>[4x]HYTWPRVNDGADWQQVRKADNWQDNGYVGDVTSPQIRCFQATPSPAPSVLNTTAGSTVTYWANPDVYHPGPVQFYMARVPDGEDINSWNGDGAVWFKVYEDHPT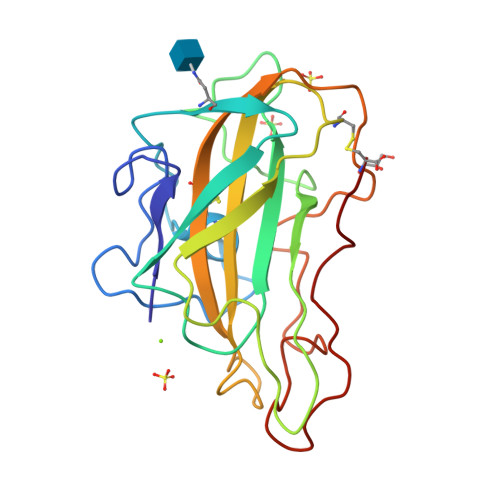FGAQLTWPSTGKSSFAVPIPPCIKSGYYLLRAEQIGLHVAQSVGGAQFYISCAQLSVTGGGSTEPPNKVAFPGAYSATDPGILINIYYPVPTSYQNPGPAVFSC> STPIQQLLEHFLRQLQRKDPHGFFAFPVTDAIAPGYSMIIKHPMDFGTMKDKIVANEYKSVT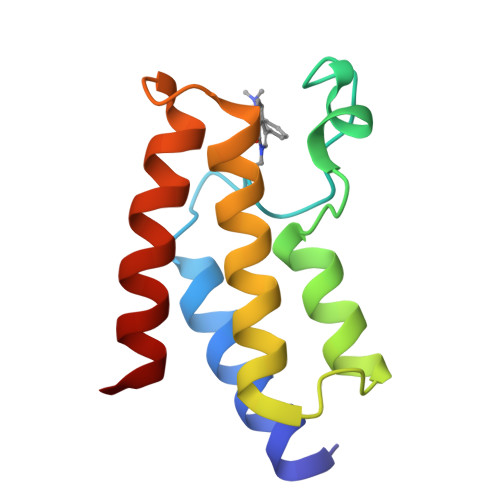EFKADFKLMCDNAMTYNRPDTVYYKLAKKILHAGFKMMSK>[12x]MAKFPKNFMFGYSWSGFQFEMGLPGSEVESDWWVWVHDKENIASGLVSGDLPENGPAYWHLYKQDHDIAEKLGMDCIRGGIEWARIFPKPTFDVKVDVEKDEEGNIISVDVPESTIKELEKIANMEALEHY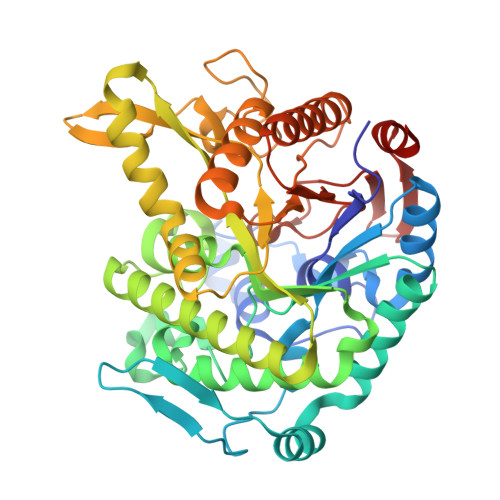RKIYSDWKERGKTFILNLYHWPLPLWIHDPIAVRKLGPDAAPAGWLDEKTVVEFVKFAAFVAYHLDDLVDMWSTMNEPNVVYNQGYINLASGFPPGFLSFEAAEKAKFNLIQAHIGAYDAIKEYSEKSVGVIYAFAWHDPLAEEYKDEVEEIRKKDYEFVTILHSKGKLDWIGVNYYSRLVYGAKDGHLVPLPGYGFMSERGGFAKSGRPASDFGWEMYPEGLENLLKYLNNAYELPMIITENGMADAADRYRPHYLVSHLKAVYNAMKEGADVRGYLHWSLTDNYEWAQGFRMRFGLVYVDFETKKRYLRPSALVSVK>[6x]GPGKTDSSFIMDSDPRRCMRHHYVDSISHPLYKCSSKMVLLARCEGHCSQASRSEPLVSFSTVLKQPFRSSCHCCRPQTSKLKALRLRCSGGMRLTATYRYILSCHCEECNSGTETSQVAPA;> EEEEEEE;> EEEE

Norrie Disease Protein (NDP) gene encodes Norrin, a secreted cystine-knot like growth factor, distinct from the lipid-modified Wnt. Unlike Wnts which have promiscuous interactions with Fz receptors, Norrin specifically binds to Fz4CRD, but not to the 14 other CRDs of Fz and secreted Frizzled-related protein (sFRP) family members. The Norrin mediated pathway maintains the blood-retina and blood-brain barriers and regulates angiogenesis in the cochlea and uterus as well as neuroprotective effects on retinal neurons. Our crystallographic and solution studies further reveal that dimeric Norrin forms a complex with two copies of monomeric Fz4CRD.

We determined three crystal structures of Norrin, using selenomethionine-labeled protein for phasing. The Norrin protein fold is identical to that of the previously reported MBP-Norrin crystal structure. Each Norrin monomer comprises three β-hairpins (β1-β2, β3-β4 and β5-β6), a β7 strand at the C-terminus, and four intramolecular disulphide bonds. The two monomers assemble as an elongated, head-to-tail, dimer stabilized by three intermolecular disulphide bridges (Cys93-Cys95, Cys95-Cys93, and Cys131-Cys131), in agreement with small-angle X-ray scattering (SAXS) measurements which showed Norrin dimer in solution. The dimer interface is further stabilized by extensive hydrogen bonds and hydrophobic interactions. Superposition of all molecules in the asymmetric units from our three crystal forms with the MBP-Norrin structure showed an average root-mean-square (r.m.s.) deviation of 1.5 Å over 190 equivalent Cα atoms. On inspection the superpositions revealed a high degree of conformational plasticity in the β1-β2, β3-β4 and β5-β6 loops. The flexibility inherent in these regions is consistent with the relatively high crystallographic B factor values. Conversely, the structural comparisons underscore the conserved nature of the interface at the dimer core.> MPRYGFHLSIAGKKGVAGAVEEATALGLTAFQIFAKSPRSWRPRALSPAEVEAFRALREASGGLPAVIHASYLVNLGAEGELWEKSVASLADDLEKAALLGVEYVVVHPGSGRPERVKEGALKALRLAGVRSRPVLLVENTAGGGEKVGARFEELAWLVADTPLQVCLDTCHAYAAGYDVAE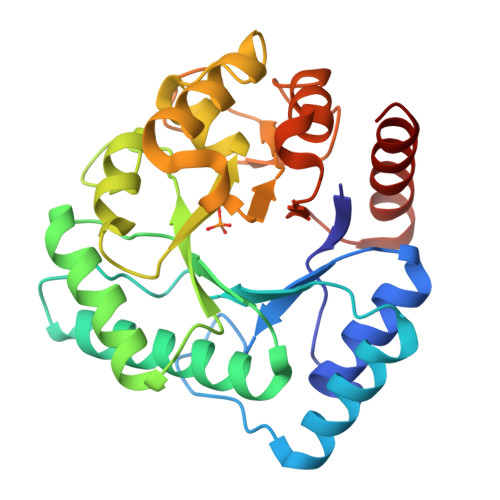DPLGVLDALDRAVGLERVPVVHLNDSVGGLGSRVDHHAHLLQGKIGEGLKRVFLDPRLKDRVFILETPRGPEEDAWNLRVFRAWLEEA> MMKAKVIDAVSFSYILRTVGDFLSEANFIVTKEGIRVSGIDPSRVVFLDIFLPSSYFEGFEVSQEKEIIGFKLEDVNDILKRVLKDDTLILSSNESKLTLTFDGEFTRSFELP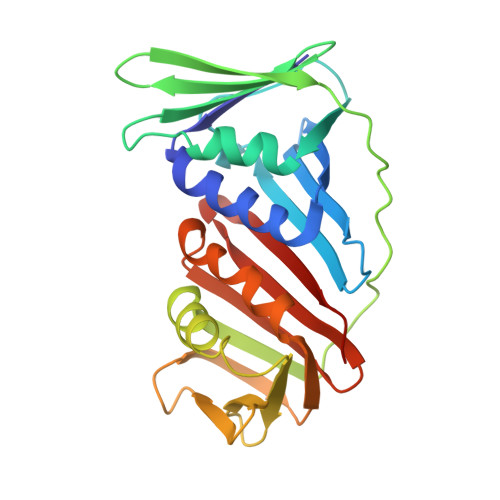LIQVESTSPPSVNLEFPFKAQLLTITFADIIDELSDLGEVLNIHSKENKLYFEVIGDLSTAKVELSTDNGTLLEASGADVSSSYGMEYVANTTKMRRASDSMELYFGSQIPLKLRFKLPQEGYGDFYIAPRAD>RPQGATVSLWETVQKWREYRRQCQRSLTEDPPPATDLFCNRTFDEYACWPDGEPGSFVNVSCPWYLPWASSVPQGHVYRFCTAEGLWLQKDNSSLPWRDLSECEESKRGERSSPEE[2x];>HXEGCFTSDVSSYLEGQAA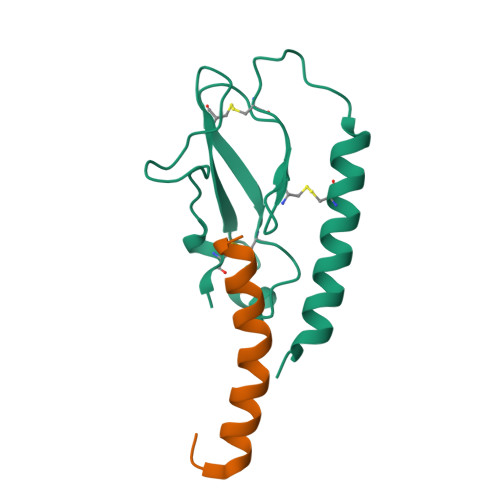KEFIAWLVKGRG[2x]> MSHHHHHHSGSGSGDKEIVEEVRKLVEEAKKRNEESNEEVKKLVEEAEEALKKAKGEEEVLKIAKEAFELAIEAAKRNLKVAKEAFELVIEAIKAITDDEAVLRLAELAAELAKSQLESLLKIAEAAMRLAASAIKAAKGDEAIVEIVRLLVEVAEEINKASNAVVKFLVEVAKEALKVAKGEEVVLEIARLAFELAIEAAKINLEVARLAFELVITAIEAITDDEAVLRLAKLAAELAKSQLESLLNIAEAAMELAASAIKAAKGDEAIVEIVRLLVEVAKEINKASNAVVEFLVEVAEEALRVAKGEEVVLEIARLAFELAIEAARINLEVARLAFELVITAIEAITDDEAVLKLAELAAELAKSQLESLLRIAEAAMRLAASAIKAAKGDEAIVEIVRLLVEVAEEINKASNAVVEFLVEVAEEALRVAKGEEVVEEIAKLAKELADEAAKINEEVAKLAEELVKTAEEAITDDEARKKLRELAKKLRKSQEESKKRIKEAAEKLEASARKAAKG

Here we describe extendable linear, curved and angled protein building blocks, as well as inter-block interactions, that conform to specified geometric standards; assemblies designed using these blocks inherit their extendability and regular interaction surfaces, enabling them to be expanded or contracted by varying the number of modules, and reinforced with secondary struts. We construct twistless helix repeat (THR) protein blocks from identical straight α-helices (typically 2–4 helices in each unit); the length of the blocks can be varied simply by varying the number of repeat units. Restricting helical geometry to ideal straight helices with zero helical twist in principle considerably limits what types of structure could be built, but this is more than compensated by the great simplification of downstream material design, as illustrated below. Using X-ray crystallography and electron microscopy, we validate nanomaterial designs ranging from simple polygonal and circular oligomers that can be concentrically nested, up to large polyhedral nanocages and unbounded straight ‘train track’ assemblies with reconfigurable sizes and geometries that can be readily blueprinted.

To generate straight, linear THRs, we set Δθ to zero. This results in perfectly straight repeat proteins in which each repeat unit is translated but not rotated relative to the previous unit. We tested 33 linear THRs (with Δh = 0) with helices either about 20 or about 40 residues in height; 23 of 33 tested designs were solubly expressed, and 13 of 19 designs analysed by SEC were primarily monomeric as designed. Structural characterization of the linear building blocks by X-ray crystallography individually and/or cryogenic EM (cryo-EM) in the context of assemblies (see below) revealed that both the detailed internal structures and the overall straight linear geometry were successfully achieved. a,b, The linear THR designs (rainbow) are nearly identical to the experimentally determined structures (grey). Right: the 2.7-Å-resolution crystal structure of the tall, linear THR5 has a 0.6 Å CA RMSD to the design. b, Bottom: Comparison of the stair-stepping linear THR4 design model to the cryo-EM structure (determined as part of a nanocage assembly).>[2x]MGSSHHHHHHSSGRENLYFQGMASIVFSTIGNPKGYQKVTYEIDGEKFESNVSVLALRDLLKVDKTVVILGISVADVYNCKYADYRSCKECIIQNSKNDLGISESYVVAPNVYQKFKGKPDHYFTYIYYHSLRILEK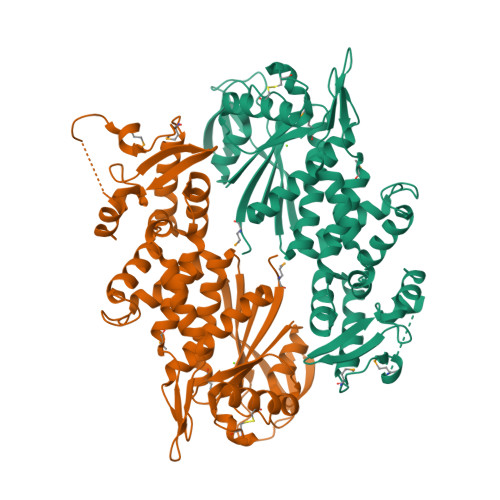EGINEVFIDTTHGINYMGVLAKEAIQLAVSAYAAKSEKEVKVSLYNSDPVGKDVSDTVKLHEIEAIKISPLSGLKYVTYQILNKDKNFFNKIFSDSVNAIPRFATALDNGLFIYLSEKDSSLHLKRLEDDLSKDPLLTPSENEINVVYKDMKYALSHALFYVISRFSGNVDLDTLRHYAETYADKVTRAIIENEVDKIEKYQMGSERKLLGEYMKVEGKGFDKRILYAHGGLPYAGTYVYKEKDKVYVTYGDKIDEIERQIGS> MAAIPPDSWQPPNVYLETSMGIIVLELYWKHAPKTCKNFAELARRGYYNGTKFHRIIKDFMIQGGDPTGTGRGGASIYGKQFEDELHPDLKFTGAGILAMANA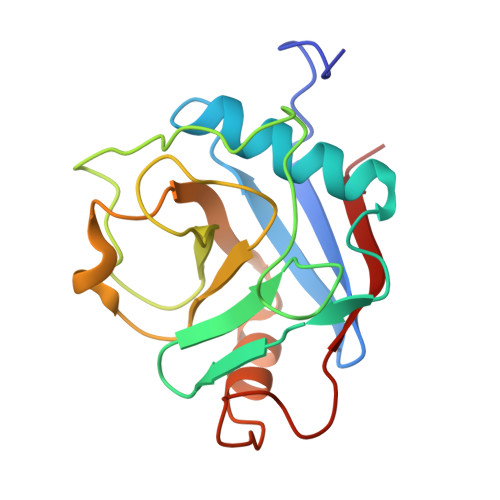GPDTNGSQFFVTLAPTQWLDGKHTIFGRVCQGIGMVNRVGMVETNSQDRPVDDVKIIKAYPSG> MTISSAHPETEPKWWKEATFYQIYPASFKDSNDDGWGDMKGIASKLEYIKELGADAIWISPFYDSPQDDMGYDIANYEKVWPTYGTNEDCFALIEKTHKLGMKFITDLVINHCSSEHEWFKESRSSKTNPKRDWFFWRPPKGYDAEGKPIPPNNWKSYFGGSAWTFDEKTQEFYLRLFCSTQPDLNWENEDCRKAIYESAVGYWLDHGVDGFRIDVGSLYSKVVGLPDAPVVDKNSTWQSSDPYTLNGPRIHEFHQEMNQFIRNRVKDGREIMTVGAMQHASD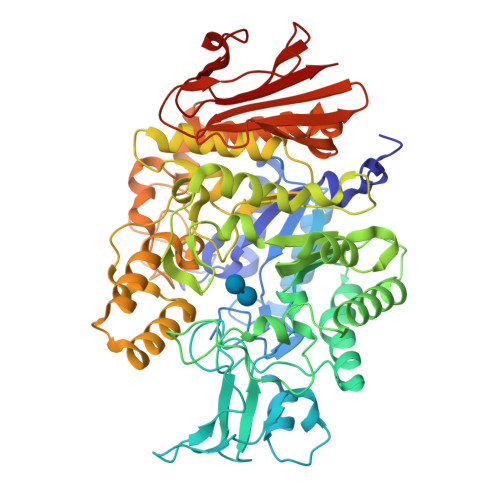ETKRLYTSASRHELSELFNFSHTDVGTSPLFRYNLVPFELKDWKIALAELFRYINGTDCWSTIYLENHDQPRSITRFGDDSPKNRVISGKLLSVLLSALTGTLYVYQGQELGQINFKNWPVEKYEDVEIRNNYNAIKEEHGENSEEMKKFLEAIALISRDHARTPMQWSREEPNAGFSGPSAKPWFYLNDSFREGINVEDEIKDPNSVLNFWKEALKFRKAHKDITVYGYDFEFIDLDNKKLFSFTKKYNNKTLFAALNFSSDATDFKIPNDDSSFKLEFGNYPKKEVDASSRTLKPWEGRIYISE> TIGMIALDAQGNLSGACTTSGMAYKMHGRVGDSPIIGAGLFVDNEIGAATATGHGEEVIRTVGTHLVVELMNQGRTPQQACKEAVERIVKIVNRRGKNLKDIQVGFIALNKKGEYGAYCIQDGFNFA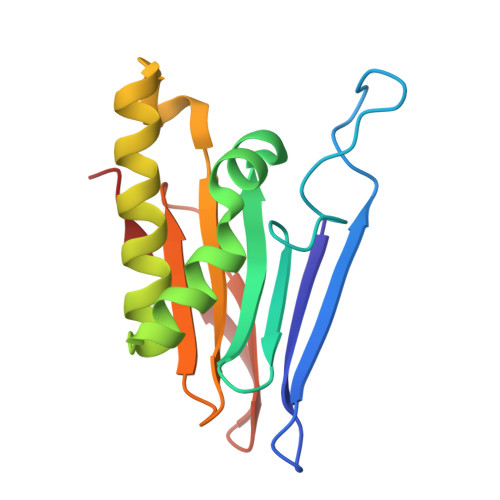VHDQKGNRLETPGFALK> STTTNSNSIGRPNLV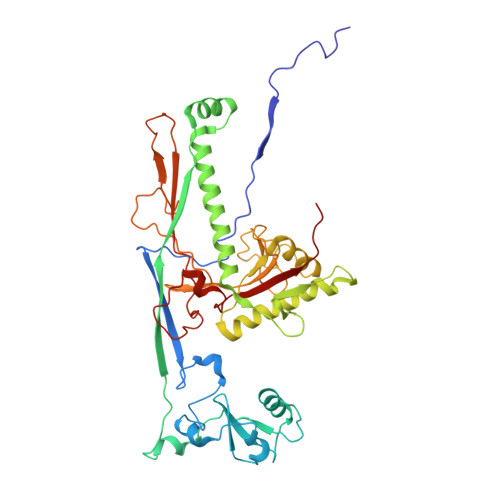ALTRATTKLIYSDIVATQRTNQPVAAFYGIKYLNPDNEFTFKTGATYAGEAGYVDREQITELTEESKLTLNKGDLFKYNNIVYKVLEDTPFATIEESDLELALQIAIVLLKVRLFSDAASTSKFESSDSEIADARFQINKWQTAVKSRKLKTGITVELAQDLEANGFDAPNFLEDLLATEMADEINKDILQSLITVSKRYKVTGITDSGFIDLSYASAPEAGRSLYRMVCEMVSHIQKESTYTATFCVASARAAAILAASGWLKHKPEDDKYLSQNAYGFLANGLPLYCDTNSPLDYVIVGVVENIGEKEIVGSIFYAPYTEGLDLDDPEHVGAFKVVVDPESLQPSIGLLVRYALSANPYTVAKDEKEARIIDGGDMDKMAGRSDLSVLLGVKLPKIII4-amino-5-hydroxy-6-[(E)-(3-{[3-(2-methylpropanoyl)pyrazolo[1,5-a]pyridin-2-yl]methyl}phenyl)diazenyl]naphthalene-1,3-disulfonic acid | C28 H25 N5 O8 S2 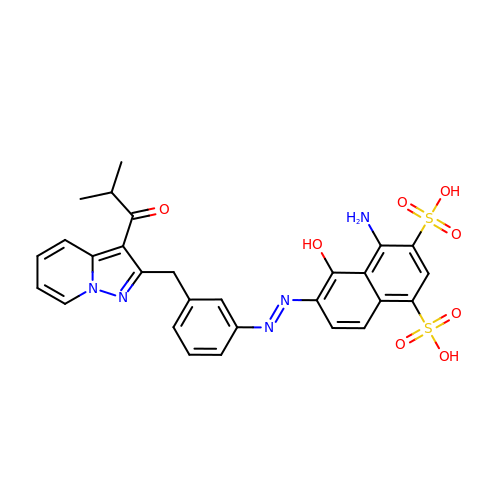| DDUSPQQMFMSMNK-NVQSTNCTSA-N>ACDYTCGSACYSSSDVSTAQAAGYKLHEDGETVGSNSYPHKYNNYEGFDFSVSSPYYEWPILSSGDVYSGGSPGADRVVFNENNQLAGV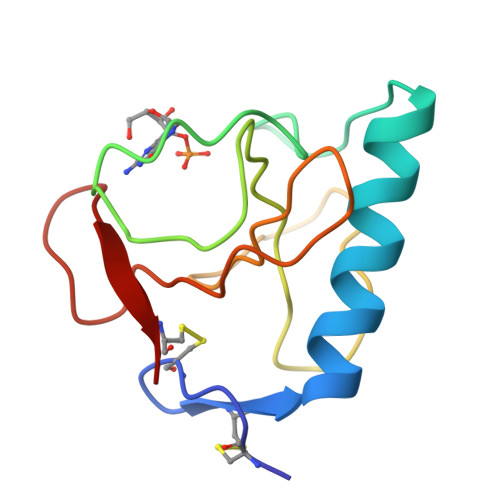ITHAGASGNNFVECT[4x]>MAHHHHHHMSTNPSLMTSFDVNKIRKDFPVLHQKINEYDLVYFDNAATTQKPKAVIDAIAQFYEKDNSNVHRGVHALSVRATEMYEAARAKVKRFINARSPRECIFVRGTTEAINLVAQSLVAPRILPDEEILITHMEHHSNIVPWQMVCKKMGCKLQVAPISLNGEVILEEFERKLNENTKMVAINYASNSLGTINPVKTMIKMAHEVGAKVLLDGAQATAHLIVDVQDLDCDFYAFSGHKMYGPTGIGVLWGKEELLNSMTPYQGGGEMINSVSFEATEYAAIPHKFEAGTPNIAGAIGLAAAIDYIWSLDLDAIAEYET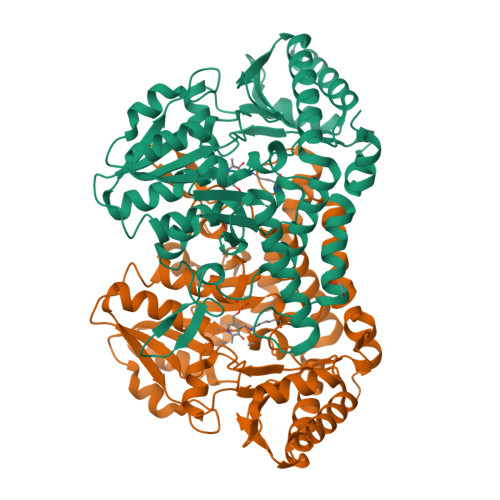QLLNYATKAIEAVKGYNIIGTAANKVPIISFVHGKIHAHDIGTILDSEGIAIRSGHHCTMPLMDFYDVAATSRISMSFYNTFKEIDYCMEALQRVKEVFA[2x]> MTSYSFTEKKRIRKDFGKQRSILEVPFLLAIQVDSYREFLQEDVESTKRKDLGLHAALKSVFPISSYSGNAALEYVGYKLGQPVFDERECRQRGMSYGAPLRVTVRLVIYDRESSTKAIKYVKEQEVYLGEIPLMTGNGTFIVNGTERVIVSQLHRSPGVFFDHDRGKTHSSGKLLYSARIIPYRGSWLDFEFDPKDALFTRIDRRRKLPVSILLRALGYNNEEMLAEFFEINTFHINPDEGVQLELVPERLRGETLNFDLADGDKVIVEAGKRITARHVKQLEAAGVAALAVPDDYLVGRILSHDVVDGSTGELLANANDEISEDQLTAFRKAGVDAVGTLWVNDLDRGPYLSNTLRIDPTKTQLEALVEIYRMMRPGEPPTKEAAQNLFHNLFFTFERYDLSTVGRMKFNRRVGRKDVLGESVLYDKKYFAERNDEESKRLVAEHTDTSDILEVIKVLTEIRNGRGVVDDIDHLGNRRVRSVGEMAENVFRVGLVRVERAVKERLSMAESEGLTPQELINAKPVAAAIKEFFGSSQLSQFMDQNNPLSEVTHKRRVSALGPGGLTRERAGFEVRDVHPTHYGRVCTIETPEGPNIGLINSLAVFARTNQYGFLETPYRKVLDGKVSDDVEYLSAIEENEYVIAQANALTDAKNMLTEQFVPCRFQGESLLKPPSEVHFMDVSPMQTVSVAAALVPFLEHDDANRALMGANMQRQAVPTLRSQKPLVGTGIERAVARDSGVTVNALRGGVIEQIDAARIVVKVNEAEIGGGTDAGVDIYNLIKYTRSNQNTCINQRPLVNVGDVIARGDVLADGPSTDIGELALGQNMLIAFMPWNGYNFEDSILLSERVVEEDRYTTIHIEELTCVARDTKLGPEEISADIPNVSEQALNRLDESGVVYIGAEVRAGDIMVGKVTPKGESQLTPEEKLLRAIFGEKASDVKDSSLRVPPGMDGTVIDVQVFTRDG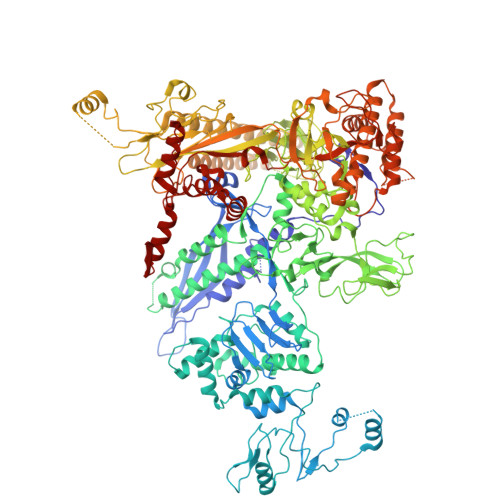IEKDKRARQIEENEIKRVKKDFDDQFRILEAAIYARLRSQIVGKVANGGANLKKGDSVTDAYLDGLKKSDWFQLRMKDEDAADAIERAQKQIQAHEKEFEARFADKRGKITQGDDLAPGVLKMVKVFLAVKRRIQPGDKMAGRHGNKGVVSNVVPVEDMPYMATGESVDIVLNPLGVPSRMNIGQILEVHLGWAAKGLGRKIQRMLEAQAAVSELRKFLDDIYNHDNAINAQRVDLSQFSDEELLNLGKNLIDGVPMATPVFDGASEAEIKRMLELADLPQSGQTQLYDGRTGEAFDRKTTVGYMHYLKLNHLVDDKMHARSTGPYSLVTQQPLGGKAQFGGQRFGEMEVWALEAYGAAYTLQEMLTVKSDDVQGRNQMYKNIVDGEHEMVAGMPESFNVLVKEIRSLAIHMELEE>[2x]SEEIQKPYKNLAKALQNPADVRNLDLSFQ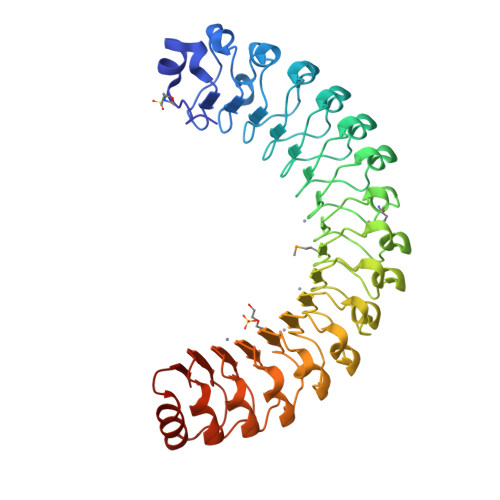GLKTLPNKIGQLKNLQKLDLGGNEPTILSKEIWQLKDLQKLNLNNNKLTVLPKEIGQLQNLQELSLHSNELVNLPKEIGQFKNLQKLNLDNNKLTVLPKEIGQLQNLQELSLLSNKLISLPTEIEQLKSLKNLDLNHNEFTTVSKEVMLLETLENLDLRSNKLKTIPKEIRQLKSLKVLMLTGNQLTSLPKEIEQLQNLKTLNLGENRFQIFPVEILELKNLLELNLYYNQLVEFPKEVGQLKSLKYLSLYHNQITTLPVEVTQLPDLQELHLSGNKITILPKEILQLKNLEWLSLSNNKLNALPKEIGQLKKLQRLELGNNQLTTLPKEIEQLKNLQRLELDSNPISPKEKERIRKLLPKCEIDFEGGGGE Found in both prokaryotes and eukaryotes, aldehyde dehydrogenases (ALDH) (EC 1.2.1.3) constitute a large family of NAD(P)-dependent enzymes with molecular weights of 50–60 kDa. ALDHTt contains an unusually extended C-terminal arm forming novel interactions with the N-terminus in the quaternary structure which interacts closely with the substrate entry tunnel. The ALDHTt monomer is composed of the three domains common to all ALDHs: (i) The NAD(P)+ binding domain (1–125 + 148–261) comprising a Rossman fold, (ii) the catalytic domain (267–458) and (iii) the oligomerization domain (126–147 + 494–501). However, the presence in ALDHTt of an unusual extended arm that wrap the facing monomer through H-bonds and salt bridges shows for the first time how the tetramer is not merely a dimer-of-dimers carrying out their functions independent of each other, but that the interaction of the N- and C-termini in CS-related monomers may regulate active site access in NCS-related molecules.

To probe the significance of the tail and its fulcrum points, two truncated tail mutants were made: (i) ALDHTt515 which removes all residues distal to the “Crook & Hook” and (ii) ALDHTt508, a mutant which removes the “Crook & Hook” entirely but retains the “Notch” to try and model other tail containing ALDHs. The co-crystal structure of ALDHTt515 was solved with NADP+ bound in the expected cofactor binding cleft of the monomeric subunit. Comparison of the NADP-bound with apo structures did not reveal significant conformational changes for the adenosine pyrophosphate accommodation within the cofactor binding cleft. The 2′-phosphate group is positioned in the ceiling of the binding cleft with O2 and O3 within 3 Å distance from Glu185 carboxyl group. While these unfavorable contacts could result in electrostatic repulsion, the 2′ phosphate is stabilized by hydrogen bonds with the Glu185 backbone amide group in addition to Ser184 and Lys182 side chains. Despite the co-crystals of the truncated mutant ALDHTt515-NADP+ being significantly larger and better diffracting than those with NAD+, enzyme kinetics data described in this work indicates that the preferential cofactor is NAD+. In addition, these data are supported by the observed proximity of the 2′ phosphate to Glu185, which gives the structural basis for NAD+ preference in ALDHTt. Indeed, in NADP-bound structures, Glu261 sidechain is in the “intermediate” conformation allowing the nicotinamide ring to sit on the bottom of the catalytic tunnel, while Cys295 is observed in the nucleophile “attacking” rotamer. Upon cofactor binding, Glu261 rolls back to make a place for the cofactor, this movement is accompanied by a local 180° flip of the main chain linker loop to bring Leu262 carbonyl group toward the carboxamide nitrogen of the nicotinamide for stabilization.

>MHHHHHHRKAAGKYGNTLEFGHLVGGEEVLEGPLLERRNPSDREDVVARFPEADKDLVRKAALKAREAFAEWSRTPAPIRGQVLFNLVKILEREKPTLTRLMVREVGKTPKEAAGDVQEAIDTALFFASEGRRLYGQTVPSEMRDKELFTFRRPLGVVGIITAGNFPIAVPSWKLIPAVLTGNTVVWKPSEDAPTLSFVFAKLFEEAGLPPGVLNVVFGGGKGSTGQWMVELMDEGLFQKFAFTGSTQVGRWIGEVAGRNLIRPTLELGGKNPLVVMRDADLDLAVEGAWWSAFATGGQRCTSAGNILVDAPIYEEFKRRFLERVEATLVGNPLLHPEVTYGPFINERFFARWQEHYRVGEAEGARLLFGRGRITRENPYPRFLGDPEAGLYGWPTVWEVRPGTRLFTEEVFGPTINLVKVDGIEEAIAVANSTPYGLSSAIYTNHRHWAYLFKVGIRAGMTSINNATVGAEAHLPFGGVKASGNGGRESGIWVLEEYTYWHAVNEEYSGRLQLAQMDTGY[2x]>SKEHMKKLMKDLEGLHRAEQSLHDLQERLHKAQEEHRTVEVEKVHLEKKLRDEINLAKQEAQRLKELREGTENERSRQKYAEEEMEQVREALRKAEKELESHSS[4x]

Two protein families are involved in this signaling pathway: the ER-localized stromal interaction molecule (STIM) calcium sensors and the calcium-release activated calcium (CRAC) channels (consisting of Orai family proteins), which are located in the plasma membrane. Next, the STIM1 oligomers rapidly migrate to ER-plasma membrane junctions, where they activate CRAC channels by directly binding to Orai1. The cytoplasmic C-terminus of STIM1 (STIM1-Ccyto, approximately 51 kDa) contains two extensive coiled-coil regions, a Pro/Ser-rich domain and a Lys-rich domain. Our recent study demonstrated that the inhibitory helix (amino acids 310-337, referred to as IH), which is close to the SOAR dimer, tightly binds to SOAR to prevent its exposure, thus keeping STIM1-Ccyto in an inactive resting state.

To better understand the conformational change of CC1 in the presence of the IH region, we determined the crystal structure of a STIM1 construct (amino acids 237-340, hereafter referred to as CC1-IH) and demonstrated the existence of both the inactive and active states of the STIM1 C-terminus in solution. One CC1-IH mutant (residues 237-340 with two mutations [M244L and L321M], referred to as CC1-IH-mut) yielded high-quality crystals that diffracted to a high resolution. The structure of CC1-IH-mut was determined using the single-wavelength anomalous dispersion (SAD) method. There are four CC1-IH-mut molecules in one asymmetric unit, and each molecule consists of an elongated α-helix stretching from its N-terminal end (referred as the head) to its C-terminal end (referred as the tail). Furthermore, two of the four CC1-IH-mut molecules have the same spatial orientation, whereas the other two are oriented in the opposite direction. As a result, all the tails of the CC1-IH-mut structure are clustered together, whereas the four heads are spread out. The two monomers paired to form the CC1-IH dimer in an antiparallel manner, with a buried surface area of 1,114.5 Å2 as calculated by AREAIMOL in the structure of CC1-IH-mut. Further structural analysis revealed that hydrophobic interactions and some intermolecular forces, such as hydrogen bonds and electrostatic attractions, are present within the interface of the dimer. These interactions mainly take place between the IH of one CC1-IH fragment and a region preceding IH in the other CC1-IH fragment. Specifically, the side chains of Leu335, Leu328, Val324 and Ala317 on one monomer (cyan) tend to exhibit hydrophobic interactions with residues Leu286, Ile290, Ala293 and Leu300 on the other monomer (green). Our current study revealed that CC1-IH exists as a long helix and that the oligomerization of CC1-IH depends on the IH domain.inosine diphosphate ribose | C15 H22 N4 O15 P2 | 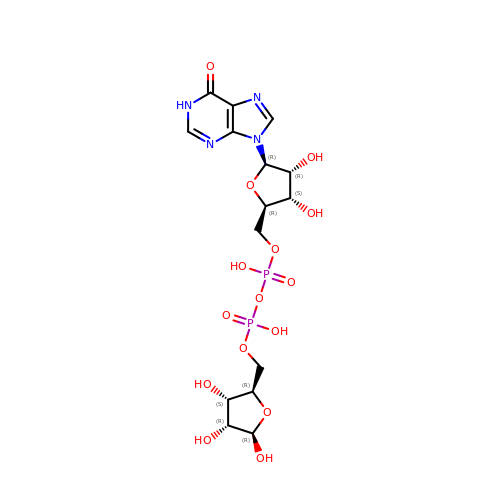GKBLKKRZILWFNP-KEOHHSTQSA-N>MITRETLKSLPANVQAPPYDIDGIKPGIVHFGVGNFFRAHEAFYVEQILEHAPDWAIVGVGLTGSDRSKKKAEEFKAQDCLYSLTETAPSGKSTVRVMGALRDYLLAPADPEAVLKHLVDPAIRIVSMTITEGGYNINETTGAFDLENAAVKADLKNPEKPSTVFGYVVEALRRRWDAGGKAFTVMSCDNLRHNGNVARKAFLGYAKARDPELAKWIEENATFPNGMVDRITPTVSAEIAKKLNAASGLDDDLPLVAEDFHQWVLEDQFADGRPPLEKAGVQMVGDVTDWEYVKIRMLNAGHVMLCFPGILVGYENVDDAIEDSELLGNLKNYLNKDVIPTLKAPSGMTLEGYRDSVISRFSNKAMSDQTLRIASDGCSKVQVFWTETVRRAIEDKRDL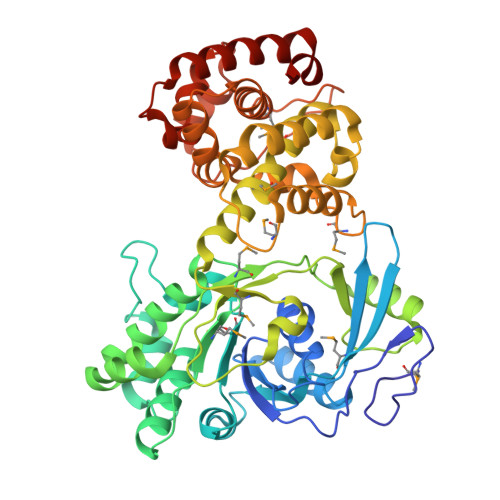SRIAFGIASYLEMLRGRDEKGGTYESSEPTYGDAEWKLAKADDFESSLKLPAFDGWRDLDTSELDQKVIVLRKIIREKGVKAAIP[2x]>[4x]ALSAEGSSGGSRGGSPKA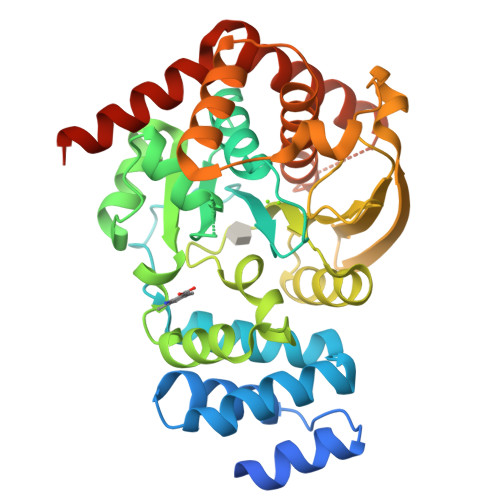EAASVPSWPQILGRLTDNRDLARGQAAWAMDQIMTGNARPAQIAAFAVAMTMKAPTADEVGELAGVMLSHAHPLPADTVPDDAVDVVGTGGDGVNTVNLSTMAAIVVAAAGVPVVKHGNRAASSLSGGADTLEALGVRIDLGPDLVARSLAEVGIGFCFAPRFHPSYRHAAAVRREIGVPTVFNLLGPLTNPARPRAGLIGCAFADLAEVMAGVFAARRSSVLVVHGDDGLDELTTTTTSTIWRVAAGSVDKLTFDPAGFGFARAQLDQLAGGDAQANAAAVRAVLGGARGPVRDAVVLNAAGAIVAHAGLSSRAEWLPAWEEGLRRASAAIDTGAAEQLLARWVRFGRQILEHHHHHH> MDERIQALRKEVDRV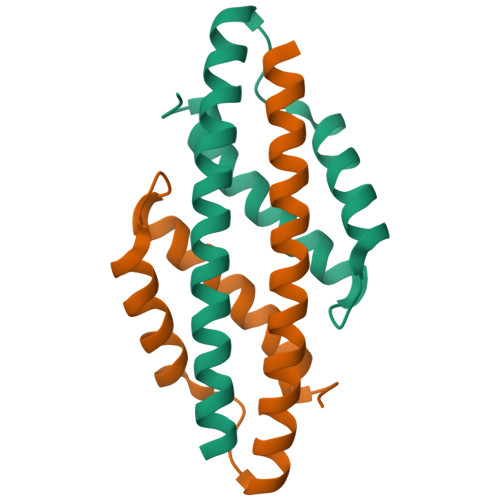NREILRLLSERGRLVQEIGRLQTELGLPHYDPKREEEMLAYLTAENPGPFPDETIRKLFKEIFKASLDLEERQDQ>MEALIPVINKLQDVFNTVGADIIQLPQIVVVGTQSSGKSSVLESLVGRDLLPRGTGIVTRRPLILQLVHVSQEDKRKTTGEENGVEAEEWGKFLHTKNKLYTDFDEIRQEIENETERISGNNKGVSPEPIHLKIFSPNVVNLTLVDLPGMTKVPVGDQPKDIELQIRELILRFISNPNSIILAVTAANTDMATSEALKISREVDPDGRRTLAVITKLDLMDAGTDAMDVLMGRVIPVKLGIIGVVNRSQLDINNKKSVTDSIRDEYAFLQKKYPSLANRNGTKYLARTLNRLLMHHIRDCLPELKTRINVLAAQYQSLLNSYGEPVDDKSATLLQLITKFATEYCNTIEGTAKYIETSELCGGARICYIFHETFGRTLESVDPLGGLNTIDILTAIRNATGP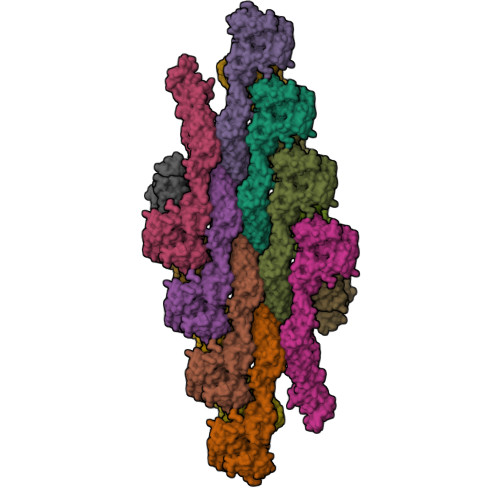RPALFVPEVSFELLVKRQIKRLEEPSLRCVELVHEEMQRIIQHCSNYSTQELLRFPKLHDAIVEVVTCLLRKRLPVTNEMVHNLVAIELAYINTKHPDFADACGLMNNNIEEQRRNRLARELPSAVSRDKLIQDSRRETKNVASGGGGVGDGVQEPTTGNWRGMLKTSKAEELLAEEKSKPIPIMPASPQKGHAVNLLDVPVPVARKLSAREQRDCEVIERLIKSYFLIVRKNIQDSVPKAVMHFLVNHVKDTLQSELVGQLYKSSLLDDLLTESEDMAQRRKEAADMLKALQGASQIIAEIRETHLW[8x];>TLQERLLAFERDRVTIPAAQVALAKQLAGDIALELQAYFRSKFPELPFGAFVPGGPLYDGLQAGAADHVRLLVPLVLEPGLWSLVPGVDTVARDPRCWAVRRTQLEFCPRGSSPWDRFLVGGYLSSRVLLELLRKALAASVNWPAIGSLLGCLIRPSMASEELLLEVQHERLELTVAVLVAVPGVDADDRLLLAWPLEGLAGNLWLQDLYPVEAARLRALDDHDAGTRRRLLLLLCAVCRGCSALGQLGRGHLTQVVLRLGEDNVDWTEEALGERFLQALELLIGSLEQASLPCHFNPSVNLFSSLREEEIDDIGYALYSGLQEPEGLL[8x]1,3-BIS-([[3-(4-{3-[3-NITRO-5-(GALACTOPYRANOSYLOXY)-BENZOYLAMINO]-PROPYL}-PIPERAZIN-1-YL)-PROPYLAMINO-3,4-DIOXO-CYCLOBUTENYL]-AMINO-ETHYL]-AMINO-CARBONYLOXY)-2-AMINO-PROPANE 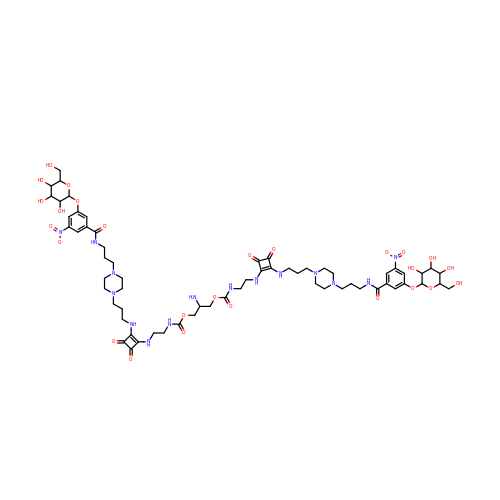| C63 H91 N15 O26 | HQTVCYHBYUXJDJ-ISUJOEFPSA-N>DKRWDQSDLHISDQTDTKGTVCSPFALFAVLENTGEKLKKSKWKWELHKLENARKPLKDGNVIEKGFVSNQIGDSLYKIETKKKMKPGIYAFKVYKPAGYPANGSTFEWSEPMRLAKCDE[3x]

Bacillus subtilis expresses TasA (translocation-dependent antimicrobial spore component) as the major biofilm protein, which aided by TapA (TasA anchoring/assembly protein, YqxM) can convert into stable oligomeric structures to form the biofilm matrix. In summary, TapA consists of an Ig domain in its core and flexible N and C termini. TapA thus functions as a chaperone in analogy to the chaperone-usher pathway since it already has a complete and especially stable V-set Ig fold and has the ability to complement TasA in the process of filament formation by donating its previously unstructured N-terminal strand. Owing to the stability of the TapA Ig domain, it is not able to open a cleft to receive a donor strand, and thus can only be located at the beginning of a filament, acting as filament inducer.

The longer construct was investigated because NMR showed long-range contacts between W74 and the core of the Ig domain. TapA71-190 shows a V-set Ig fold (InterPro code: IPR013106) composed of two antiparallel β-sheets. D71 forms four hydrogen bonds involving residues G169, W74, and R73. W74 and D71 together stabilize the loop between β-strands 8 and 9. The additional hydrogen bonding suggests a higher stability of TapA71-190, which is supported by the TSA data (Tm = 60 °C for TapA71-190 and 46 °C for TapA75-190). Structural integrity is supported by a disulfide bond linking C92 and C188. Intriguingly, the secondary structure pattern of the Ig domain resembles in its core (gray background) that of the TasA filament structure and the proteins of the chaperone-usher pathway. The high melting point of TapA (64 °C), together with the fact that it already consists of a complete Ig fold, explains its inability to be located within a filament.(4R,22R)-5,21-dioxo-4,22-bis({3-[4-(4-phenylthiophen-2-yl)phenyl]propanoyl}amino)-10,13,16-trioxa-6,20-diazapentacosane-1,25-dioic acid | C58 H66 N4 O11 S2 | 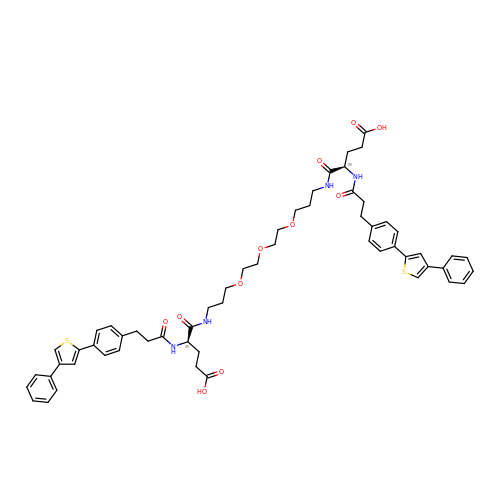PAOWMYIFDMOPGM-CDKYPKJRSA-N Complement, contact activation, coagulation, and fibrinolysis are serum protein cascades that need strict regulation to maintain human health. Serum glycoprotein, a C1 inhibitor (C1-INH), is a key regulator (inhibitor) of serine proteases of all the above-mentioned pathways. The mode of inhibition of these proteases involves interaction between the reactive center loop (RCL) of the C-terminal serpin domain of C1-INH to form a covalently linked acyl-enzyme complex that distorts the enzyme active site and is irreversibly bound. While the mechanisms of action of BrkA, BapC, and FHA are still unclear, Vag8, a 95-kDa autotransporter protein, was recently shown to interfere with the complement and contact systems by binding to C1-INH, leading to bacterial complement evasion. Autotransporters represent the type V bacterial secretion system and possess a C-terminal membrane-embedded β-barrel domain that facilitates the translocation of the N-terminal passenger domain, responsible for effector functions, across the outer membrane.

To that end, we have determined the structure of the Vag8 passenger domain in complex with the C1-INH serpin domain using single-particle cryo-electron microscopy (cryo-EM) to a resolution of 3.6 Å. A de novo model was built manually using the program COOT for the region from position 54 to 481 of Vag8. The model of the active form of the C1-INH serpin domain was placed and remodeled to fit the volume, with the only major changes in conformation being within the RCL, which is seen to be sequestered within the cleft of the Vag8 beta-barrel fold. The model for the complex reveals that C1-INH associates with the cleft within the Vag8 passenger domain beta-barrel, with two contact sites. The first involves contacts between two loops at the base of the C1-INH serpin domain (around residues 317 and 362) and one of the longer loops incorporated in the Vag8 beta barrel (residues 407 to 410). The other point of contact is a much more significant interaction which buries the side chains of the majority of the RCL residues between 461 and 474 within the Vag8 beta-barrel cleft, burying ∼600 Å2 on both components. With the exception of a mutation designed to sterically block binding of the RCL in the cleft by replacement of a small alanine side chain with a very large arginine side chain (A231R) (also data not shown), mutation of multiple residues within the cleft to alanine was required to prevent formation of the complex, emphasizing the extended nature of the interaction site. Unlike the native function of C1-INH, which results in formation of a covalent link between the RCL and the target, the inhibitor complex buries the RCL within the cleft of the bacterial protein via noncovalent interactions. Formation of a stable complex involving the RCL sterically occludes C1-INH interactions with its physiological partners.

> PTIQPTQPTTQLPTDSPTQPTTGSFCPGPVTLCSDLESHSTEAVLGDALVDFSLKLYHAFSAMKKVETNMAFSPFSIASLLTQVLLGAGENTKTNLESILSYPKDFTCVHQALKGFTTKGVTSVSQIFHSPDLAIRDTFVNASRTLYSSSPRVLSNNSDANLELINTWVAKNTNNKISRLLDSLPSDTRLVLLNAIYLSAKWKTTFDPKKTRMEPFHFKNSVIKVPMMNSKKYPVAHFIDQTLKAKVGQLQLSHNLSLVILVPQNLKHRLEDMEQALSPSVFKAIMEKLEMSKFQPTLLTLPRIKVTTSQDMLSIMEKLEFFDFSYDLNLCGLTEDPDLQVSAMQHQTVLELTETGVEAAAASAISVARTLLVFEVQQPFLFVLWDQQHKFPVFMGRVYDPRA;> AVTAAQRIDGGAAFLGDVAIATTKASEHGINVTGRTAEVRVTGGTIRTSGNQAQGLRVGTENAPDNTAVVASVFLQNLIIETSGTGALGVSVHEPQGGGGTRLSMSGTTVRTRGDDSFALQLSGPASATLNDVALETAGQQAPAVVLWQGAQLNAQGLVVQVNGAGVSAIHAQDAGSFTLSGSDITARGLEVVGIYVQEGMQGTLTGTRVTTQGDTAPALQVEDAGTHVSMNGGALSTSGANSPAAWLLAGGSAQFRDTVLRTVGEASHGVDVAAHSEVELAHAQVRADGQGAHGLVVTRSSAMVRAGSLVESTGDGAAALLESGHLTVDGSVVHGHGAAGLEVDGESNVSLLNGARLSSDQPTAIRLIDPRSVLNLDIKDRAQLLGDIAPEAQQPDGSPEQARVRVALADGGTWAGRTDGAVHTVRLLDRGVWTVTGDSRVAEVKLEGGTLAFAPPAQPKGAFKTLVATQGISGTGTIVMNAHLPSGTADVLVAPQGFGDRQVLVVNNTDDGTESGATKVPLIEDEQGHTAFTLGNMGGRVDAGARQYELTASEAQADKARTWQLTPTNELSTTATAAVNAMAIAASQRIWQAEMDVLLRHMSGLHSIGSPGGFWARGLSQRQRLDTGYGPWQKQTVSGIELGLDRRVAGGATTAWSVGMLAGYSETRRDGGAYRAGHVHSAHVGAYVSYLNDSGSYVDGVVKYNRFRHGFDIRTTDLKRVDAKHRSHGLGALLRGGRRIDIDGGWYVEPQASVAWFHAGGSRYEASNGLRVRADGAHSWVLRAGAEAGRQMRLANGNIVEPYARLGWAQELGADNAVYTNGIRHVTRSRGGFAEARVGVGALLGKRHALYADYEYAKGARFEAPWTLQLGYRYSW> DNSNGSTIPSSITSGSIFDLEGDNPNPLVDDSTLVFVPLEAQHITPNGNGWRHEYKVKESLRVAMTQTYEVFEATVKVEMSDGGKTIISQHHASDTGTISKVYVSDTDESGFNDSVANNGIFDVYVRLRNTSGNEEKFALGTMTSGETFNLRVVNNYGDVEVTAFGNSFGIPVEDDSQSYFKFGN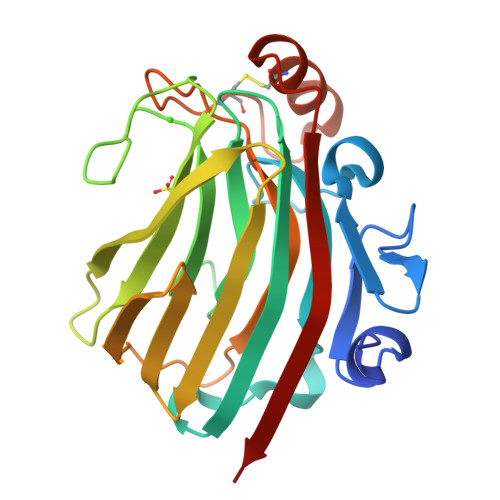YLQSQDPYTLDKCGEAGNSNSFKNCFEDLGITESKVTMTNVTYTRETN>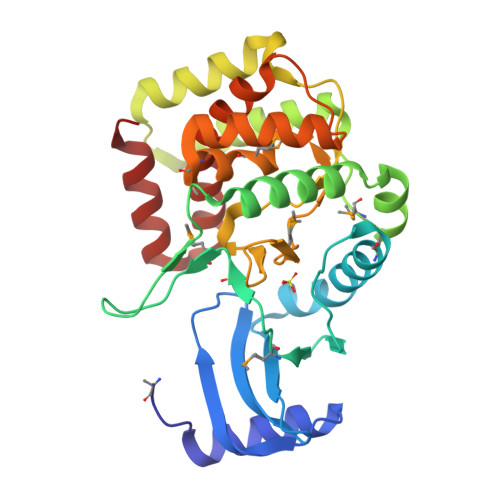 MTVVTTADTSQLYALAARHGLKLHGPLTVNELGLDYRIVIATVDDGRRWVLRIPRRAEVSAKVEPEARVLAMLKNRLPFAVPDWRVANAELVAYPMLEDSTAMVIQPGSSTPDWVVPQDSEVFAESFATALAALHAVPISAAVDAGMLIRTPTQARQKVADDVDRVRREFVVNDKRLHRWQRWLDDDSSWPDFSVVVHGDLYVGHVLIDNTERVSGMIDWSEARVDDPAIDMAAHLMVFGEEGLAKLLLTYEAAGGRVWPRLAHHIAERLAFGAVTYALFALDSGNEEYLAAAKAQLAAAE> METFDPTELPELLKLYYRRLFPYSQYYRWLNYGGVIKNYFQHREFSFTLKDDIYIRYQSFNNQSDLEKEMQKMNPYKIDIGAVYSHRPNQHNTVKLGAFQAQEKELVFDIDMTDYDDVRRCCSSADICPKCWTLMTMAIRIIDRALKEDFGFKHRLWVYSGRRGVHCWVCDESVRKLSSAVRSGIVEYLSLVKGGQDVKKKVHLSEKIHPFIRKSINIIKKYFEEYALVNQDILENKESWDKILALVPETIHDELQQSFQKSHNSLQRWEHLKKVASRYQNNIKNDKYGPWLEWEIMLQYCFPRLDINVSKGINHLLKSPFSVHPKTGRISVPIDLQKVDQFDPFTVPTISFICRELDAISTNEEEKEENEAESDVKHRTRDYKKTSLAPYVKVFEHFLENLDKSRKG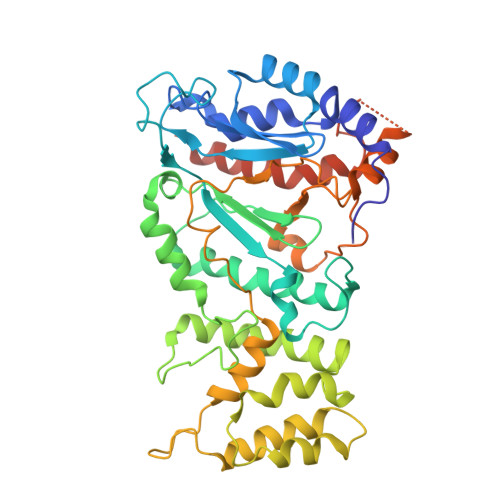ELLKKSDLQKDF>[2x]MADIYPLGKTHTEELNEIIVESAKEIAEPDTTMIQKLIDEHNPEPLLKGVRYYMCENDIEKKRRTYYDAAGQQLVDD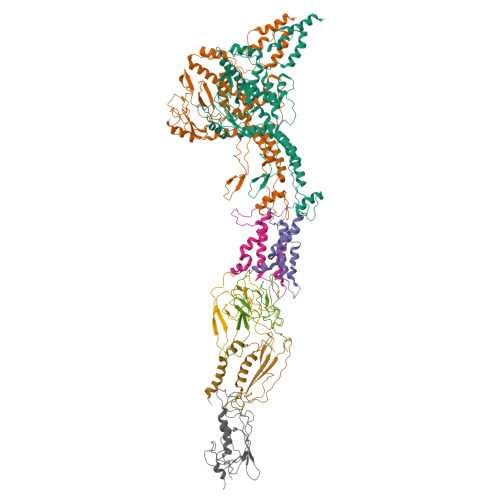TKTNNRTSHAWHKLFVDQKTQYLVGEPVTFTSDNKTLLEYVNELADDDFDDILNETVKNMSNKGIEYWHPFVDEEGEFDYVIFPAEEMIVVYKDNTRRDILFALRYYSYKGIMGEETQKAELYTDTHVYYYEKIDGVYQMDYSYGENNPRPHMTKGGQAIGWGRVPIIPFKNNEEMVSDLKFYKDLIDNYDSITSSTMDSFSDFQQIVYVLKNYDGENPKEFTANLRYHSVIKVSGDGGVDTLRAEIPVDSAAKELERIQDELYKSAQAVDNSPETIGGGATGPALEKLYALLDLKANMAERKIRAGLRLFFWFFAEYLRNTGKGDFNPDKELTMTFTRTRIQNDSEIVQSLVQGVTGGIMSKETAVARNPFVQDPEEELARIEEEMNQYAEMQGNLLDDEGGDDDLEEDDPNAGAAESGGAGQVS;>MDIQRVKRLLSITNDKHDEYLTEMVPLLVEFAKDECHNPFIDKDGNESIPSGVLIFVAKAAQFYMTNAGLTGRSMDTVSYNFATEIPSTILKKLNPYRKMAR[2x];>[2x]MYEEFRDVITFQSYVEQSNGEGGKTYKWVDEFTAAAHVQPISQEEYYKAQQLQTPIGYNIYTPYDDRIDKKMRVIYRGKIVTFIGDPVDLSGLQEITRIKGKEDGAYVG;> MTWKLASRALQKATVENLESYQPLMEMVNQVTESPGKDDPYPYVVIGDQSSTPFETKSSFGENITMDFHVWGGTTRAEAQDISSRVLEALTYKPLMFEGFTFVAKKLVLAQVITDTDGVTKHGIIKVRFTINNN;> MPETPIMGQDVKYLFQSIDAATGSAPLFPAYQTDGSVSGERELFDEQTKNGRILGPGSVADSGEVTYYGKRGDAGQKAIEDAYQNGKQIKFWRVDTVKNENDKYDAQFGFAYIESREYSDGVEGAVEISISLQVIGELKNGEIDTLPEEIVNVSKGGYDFQQPGQTTGEAPGTVPAP> MYGLVNKAIQDMISKHHGEDTWEAIKQKAGLEDIDFFVGMEAYSDDVTYHLWGAASEVLGKPAEELWIAFGEYWVTYTS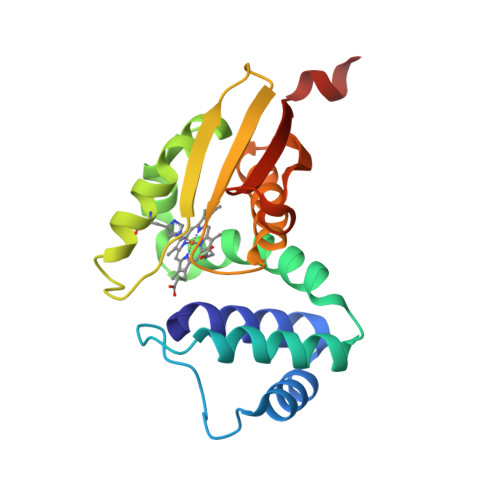EEGYGELLASAGDSLPEFMENLDNLHARVGLSFPQLRPPAFECQHTSSKSMELHYQSTRCGLAPMVLGLLHGLGKRFQTKVEVTQTAFRETGEDHDIFSIKYEGAENLYFQ> EKVAVETSVYLSELEWKSASTGYGE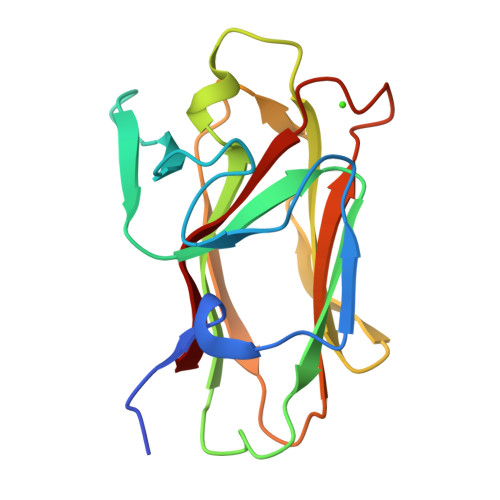IQKDASCDGNTITLKGENGEKVSYDKGIGTHAHSEIVYSLEGLDYYDYFETFVGVDQEMAGTVASISFEVYLDNEKVFDSGLMTGDTTQKHVKVPIAGKNTLKLVVKDGGDSIGSDHGSFGDAKLT> PISPIETVPVKLKPGMDGPKVKQWPLTEEKIKALVEICTEMEKEGKISKIGPENPYNTPVFAIKKKDSTKWRKLVDFRELNKRTQDFWEVQLGIPHPAGLKKKKSVTVLDVGDAYFSVPLDEDFRKYTAFTIPSINNETPGIRYQYNVLPQGWKGSPAIFQSSMTKILEPFRKQNPDIVIYQYMDDLYVGSDLEIGQHRTKIEELRQHLLRWGLTTPDKKHQKEPPFLWMGYELHPDKWTVQPIVLPEKDSWTVNDICKLVGKLNWASQIYPGIKVRQLSKLLRGTKALTEVIPLTEEAELELAENREILKEPVHGVYYDPSKDLIAEIQKQGQGQWTYQIYQEPFKNLKTGKYARMRGAHTNDVKQLTEAVQKITTESIVIWGKTPKFKLPIQKETWETWWTEYWQATWIPEWEFVNTPPLVKLWYQLEKEPIVGAETFYVDGAANRETKLGKAGYVTNRGRQKVVT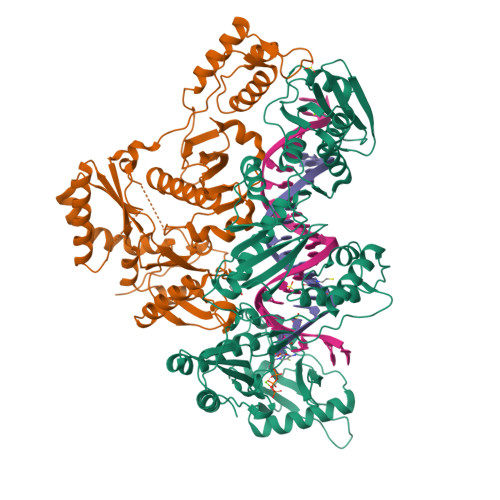LTDTTNQKTELQAIYLALQDSGLEVNIVTDSQYALGIIQAQPDQSESELVNQIIEQLIKKEKVYLAWVPAHKGIGGNEQVDKLVSAGIRK;> MGSSHHHHHHSSPISPIETVPVKLKPGMDGPKVKQWPLTEEKIKALVEICTEMEKEGKISKIGPENPYNTPVFAIKKKDSTKWRKLVDFRELNKRTQDFWEVQLGIPHPAGLKKKKSVTVLDVGDAYFSVPLDEDFRKYTAFTIPSINNETPGIRYQYNVLPQGWKGSPAIFQSSMTKILEPFRKQNPDIVIYQYMDDLYVGSDLEIGQHRTKIEELRQHLLRWGLTTPDKKHQKEPPFLWMGYELHPDKWTVQPIVLPEKDSWTVNDIQKLVGKLNWASQIYPGIKVRQLSKLLRGTKALTEVIPLTEEAELELAENREILKEPVHGVYYDPSKDLIAEIQKQGQGQWTYQIYQEPFKNLKTGKYARMRGAHTNDVKQLTEAVQKITTESIVIWGKTPKFKLPIQKETWETWWTEYWQATWIPEWEFVNTPPLVKLWYQLEKEPIVGAETF> SRLVEPYLDGYATSNVTTQIGTHAYLPCRVKQLGNKSVSWIRLRDGHILTVDRAVFIADQRFLAIKQPDKYWTLQIKYVQARDAGSYECQVSTEPKVSARVQLQVVVPHHHH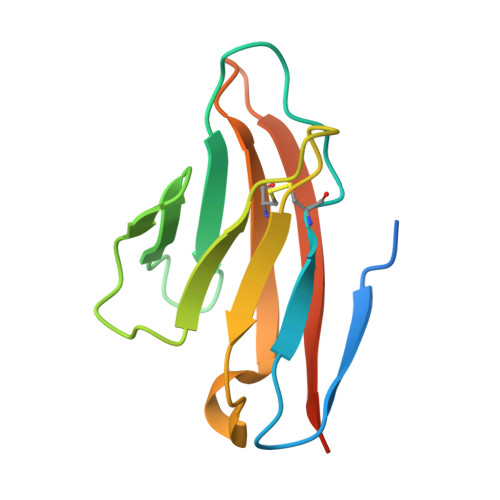HH> MDLMAYWLCITNEDNWKVIKEKKIWGVAERYKNTINKV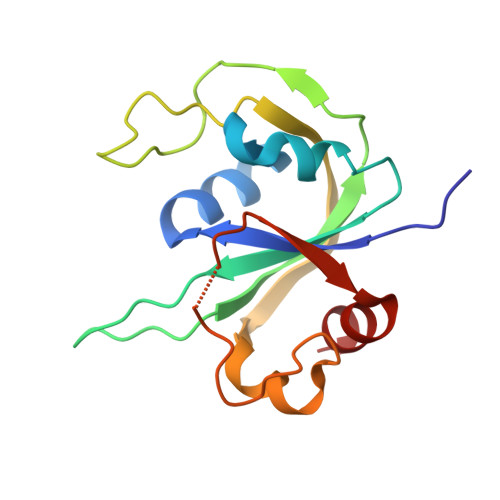KVGDKLIIYEIQRSGKDYKPPYIRGVYEVVSEVYKDSSKIFKPTPRNPNEKFPYRVKLKEIKVFEPPINFKELIPKLKFITNKKRWSGHLMGKAMREIPEEDYKLIVGN KdpFABC is a high-affinity prokaryotic K+ uptake system that forms a functional chimera between a channel-like subunit (KdpA) and a P-type ATPase (KdpB). The heterotetrametric KdpFABC complex comprises four subunits, namely the channel-like KdpA, a member of the superfamily of K+ transporters (SKT), the P-type ATPase KdpB, the lipid-like stabilizer KdpF, and KdpC, whose function is still unknown. At high K+ levels, KdpFABC needs to be inhibited to prevent excessive K+ accumulation to the point of toxicity. This is achieved by a phosphorylation of the serine residue in the TGES162 motif in the A domain of the pump subunit KdpB (KdpBS162-P).

While the first two structures represent known states of the catalytic cycle, the third KdpFABS162-PC structure obtained under turnover conditions shows an unusual compact conformation of the cytosolic domains not yet observed in the Post-Albers cycle of other P-type ATPases. The structure was resolved at an overall resolution of 3.4 Å and derived from ~14% of the initial particle set. Strikingly, the N domain is closely associated with the A domain, thereby disrupting the nucleotide-binding site between the N and P domains. Closer inspection of the nucleotide-binding site shows that the catalytic aspartate KdpBD307 is phosphorylated, but not located in proximity to the TGES162 loop of the A domain. This indicates that the state is adopted after the canonical E1P state, which, in a normal, non-inhibited catalytic cycle, would transition into an E2P state. Due to its compact organization, we termed this state E1P tight. The E1P tight state features a tilt of the A domain by 26° in helix 4 (KdpB198–208) that is not found in the other E1 states, including the E1 apo tight state (C – arrow 1). By contrast, the D307KTG loop is largely uncoiled in the E1P tight state, with the phosphorylated KdpBD307 pointing in the opposite direction, releasing this electrostatic strain. This orientation is further stabilized by a salt bridge formed with KdpBK499. We suggest that this state represents the biochemically described E1P inhibited state, and is adopted after ADP release from the high-energy E1P state, when KdpFABC attempts to relax into the E2P state (transition 4b).

> MAAQGFLLIATFLLVLMVLARPLGSGLARLINDIPLPGTTGVERVLFRALGVSDREMNWKQYLCAILGLNMLGLAVLFFMLLGQHYLPLNPQQLPGLSWDLALNTAVSFVTNTNWQSYSGETTLSYFSQMAGLTVQNFLSAASGIAVIFALIRAFTRQSMSTLGNAWVDLLRITLWVLVPVALLIALFFIQQGALQNFLPYQAVNTVEGAQQLLPMGPVASQEAIKMLGTNGGGFFNANSSHPFENPTALTNFVQMLAIFLIPTALCFAFGEVMGDRRQGRMLLWAMSVIFVICVGVVMWAEVQGNPHLLALGTDSSINMEGKESRFGVLVSSLFAVVTTAASCGAVIAMHDSFTALGGMVPMWLMQIGEVVFGGVGSGLYGMMLFVLLAVFIAGLMIGRTPEYLGKKIDVREMKLTALAILVTPTLVLMGAALAMMTDAGRSAMLNPGPHGFSEVLYAVSSAANNNGSAFAGLSANSPFWNCLLAFCMFVGRFGVIIPVMAIAGSLVSKKSQAASSGTLPTHGPLFVGLLIGTVLLVGALTFIPALALGPVAEYLS;> MSRKQLALFEPTLVVQALKEAVKKLNPQAQWRNPVMFIVWIGSLLTTCISIAMASGAMPGNALFSAAISGWLWITVLFANFAEALAEGRSKAQANSLKGVKKTAFARKLREPKYGAAADKVPADQLRKGDIVLVEAGDIIPCDGEVIEGGASVDESAITGESAPVIRESGGDFASVTGGTRILSDWLVIECSVNPGETFLDRMIAMVEGAQRRKTPNEIALTILLIALTIVFLLATATLWPFSAWGGNAVSVTVLVALLVCLIPTTIGGLLSAIGVAGMSRMLGANVIATSGRAVEAAGDVDVLLLDKTGTITLGNRQASEFIPAQGVDEKTLADAAQLASLADETPEGRSIVILAKQRFNLRERDVQSLHATFVPFTAQSRMSGINIDNRMIRKGSVDAIRRHVEANGGHFPTDVDQKVDQVARQGATPLVVVEGSRVLGVIALKDIVKGGIKERFAQLRKMGIKTVMITGDNRLTAAAIAAEAGVDDFLAEATPEAKLALIRQYQAEGRLVAMTGDGTNDAPALAQADVAVAMNSGTQAAKEAGNMVDLDSNPTKLIEVVHIGKQMLMTRGSLTTFSIANDVAKYFAIIPAAFAATYPQLNALNIMCLHSPDSAILSAVIFNALIIVFLIPLALKGVSYKPLTASAMLRRNLWIYGLGGLLVPFIGIKVIDLLLTVCGLV;> MSGLRPALSTFIFLLLITGGVYPLLTTVLGQWWFPWQANGSLIREGDTVRGSALIGQNFTGNGYFHGRPSATAEMPYNPQASGGSNLAVSNPELDKLIAARVAALRAANPDASASVPVELVTASASGLDNNITPQAAAWQIPRVAKARNLSVEQLTQLIAKYSQQPLVKYIGQPVVNIVELNLALDKLDE;> MSAGVITGVLLVFLLLGYLVYALINAE>ANPLYQKHIISINDLSRDDLNLVLATAAKLKANPQPELLKHKVIASCFFEASTRTRLSFETSMHRLGASVVGFSDSANTSLGKKGETLADTISVISTYVDAIVMRHPQEGAARLATEFSGNVPVLNAGDGSNQHPTQTLLDLFTIQETQGRLDNLHVAMVGDLKYGRTVHSLTQALAKFDGNRFYFIAPDALAMPQYILDMLDEKGIAWSLHSSIEEVMAEVDILYMTRVQKERLDPSEYANVNAQFVLRASDLHNAKANMKVLHPLPRVDEIATDVDKTPHAWYFQQAGNGIFARQALLALVLNRDLVL[2x];>[2x]MTHDNKLQVEAIKRGTVIDHIPAQIGFKLLSLFKLTETDQRITIGLNLPSGEMGRKDLIKIENTFLSEDQVDQLALYAPQATVNRIDNYEVVGKSRPSLPERIDNVLVCPNSNCISHAEPVSSSFAVRKRANDIALKCKYCEK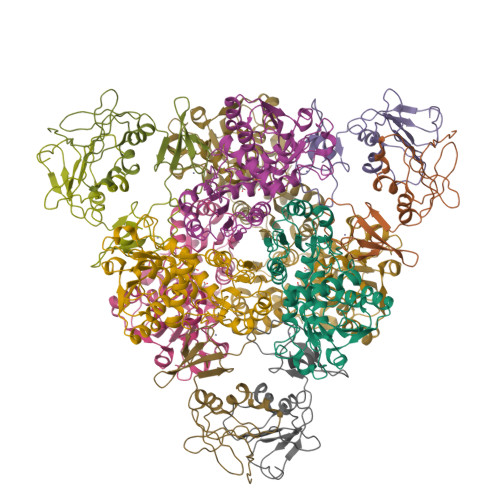EFSHNVVLAN>MADVMLNTDQINKVPNDIVTRLVRESLAEDIATGDITAQLAEDIDTTAFCITREEMILCGQDFANEVINQLDKNIQITWLYSDAQKVPANARIFELKGNVRSILTAERTILNFIQMLSGTATVTNKLVKLISQYKTKLLDTRKTIPGFRLA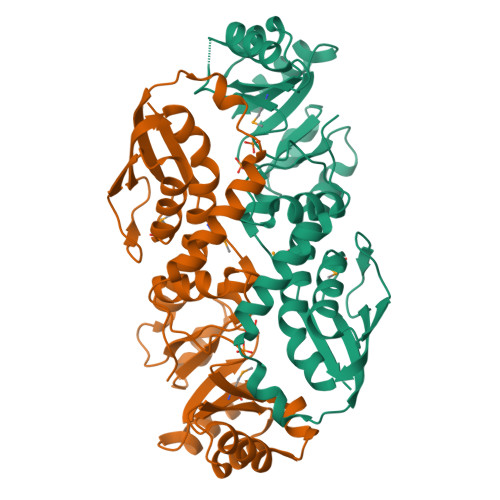QKYAVRCGGGFNHRIGLFDAYLIKENHIRSAGGIAKAVTKAKKLDSNKVVEVEVTNLDELNQAIAAKADIVMLDNFSGEDIDIAVSIARGKVALEVSGNIDRNSIVAIAKTGVDFISVGAITKHIKAIDLSLQVQL[2x]> GSKHDGRVKIGHYVLGDTLGVGTFGKVKIGEHQLTGHKVAVKILNR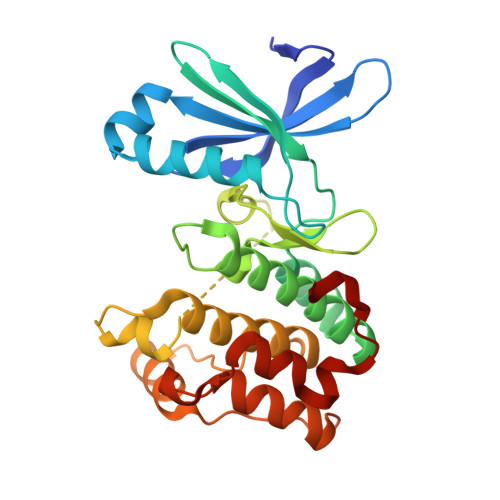QKIRSLDVVGKIKREIQNLKLFRHPHIIKLYQVISTPTDFFMVMEYVSGGELFDYICKHGRVEEMEARRLFQQILSAVDYCHRHMVVHRDLKPENVLLDAHMNAKIADFGLSNMMSDGEFLRTSCGSPNYAAPEVISGRLYAGPEVDIWSCGVILYALLCGTLPFDDEHVPTLFKKIRGGVFYIPEYLNRSVATLLMHMLQVDPLKRATIKDIREHEWFKQDLPSYLFPE> ADTLDNVNLVSSPVHSGFLVSFMVDARGGSMRGSRHHGMRIIIPPRKCTAPTRITCRLVKRHK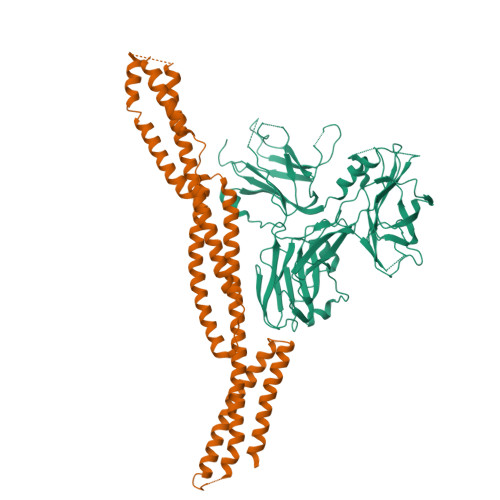LANPPPMVEGEGLASRLVEMGPAGAQFLGPVIVEIPHFGSMRGKERELIVLRSENGETWKEHQFDSKNEDLSELLNGMDEELDSPEELGTKRICRIITKDFPQYFAVVSRIKQESNQIGPEGGILSSTTVPLVQASFPEGALTKRIRVGLQAQPVPEETVKKILGNKATFSPIVTVEPRRRKFHKPITMTIPVPPPSGEGVSNGYKGDTTPSLRLLCSITGGTSPAQWEDITGTTPLTFIKDCVSFTTNVSARFWLADCHQVLETVGLASQLYRELICVPYMAKFVVFAKTNDPVESSLRCFCMTDDRVDKTLEQQENFEEVARSKDIEVLEGKPIYVDCYGNLAPLTKGGQQLVFNFYSFKENRLPFSIKVRDTSQEPCGRLSFLKEPKTTKGLPQTAVCNLNITLPAHKKAEKADRRQSFTSLALR;> AFQVEQYYFDVAEVEAWLGEQELLMMSEDKGKDEQSTLQLLKKHLQLEQGVENYEESIAQLSRQCRALLEMGHPDSEQISRRQSQVDRLYVALKELGEERRVSLEQQYWLYQLSRQVDELEHWIAEKEVVAGSPELGQDFEHVSVLQEKFSEFASETGTAGRERLAAVNQMVDELIECGHTAAATMAEWKDGLNEAWAELLELMGTRAQLLAASRELHKFFSDARELQGQIEEKRRRLPRLTAPPEPRPSASSMQRTLRAFEHDLQLLVSQVRQLQEGAAQLRTVYAGEHAEAIASREQEVLQGWKELLAACEDARLHVSST>[2x]MDEFEMIKRNTSEIISEEELREVLKKDEKSARIGFEPSGKIHLGHYLQIKKMIDLQNAGFDIIIYLADLGAYLNQKGELDEIRKIGDYNKKVFEAMGLKAKYVYGSENCLDK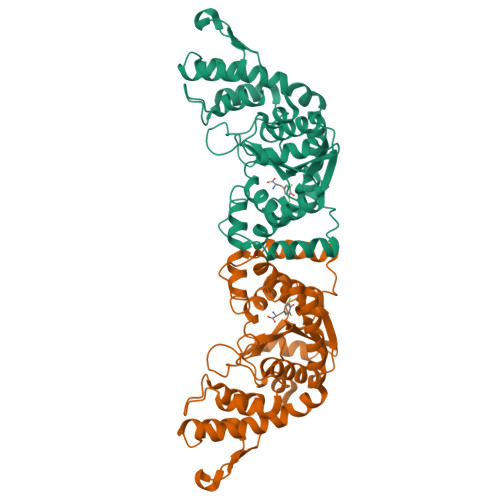DYTLNVYRLALKTTLKRARRSMELIAREDENPKVAEVIYPIMQVNNIHYSGVDVAVGGMEQRKIHMLARELLPKKVVCIHNPVLTGLDGEGKMSSSKGNFIAVDDSPEEIRAKIKKAYCPAGVVEGNPIMEIAKYFLEYPLTIKRPEKFGGDLTVNSYEELESLFKNKELHPMDLKNAVAEELIKILEPIRKRLLEHHHHHH N6-Methyladenosine 5'-triphosphate 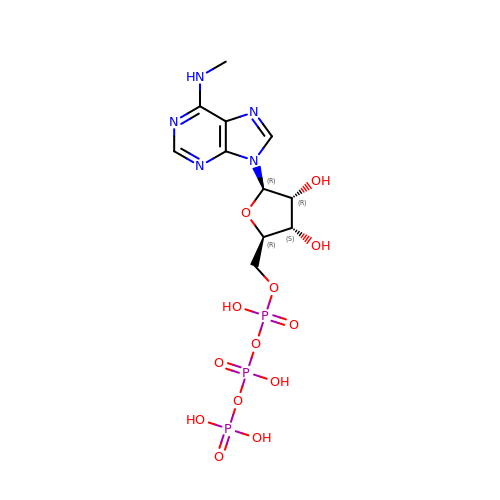| C11 H18 N5 O13 P3 | LCQWKKZWHQFOAH-IOSLPCCCSA-N> KMAFTLADRVTEEMLADKAALVVEVVEENYHDAPIVGIAVVNEHGRFFLRPETALADPQFVAWLGDETKKKSMFDSKRAAVALKWKGIELCGVSFDLLLAAYLLDPAQGVDDVAAAAKMKQYEAVRPDEAVYGKGAKRAVPDEPVLAEHLVRKAAAIWALERPFLDELRRNEQDRLLVELEQPLSSILAEMEFAGVKVDTKRLEQMGEELAEQLRTVEQRIYELAGQEFNINSPKQLGVILFEKLQLPVLKKS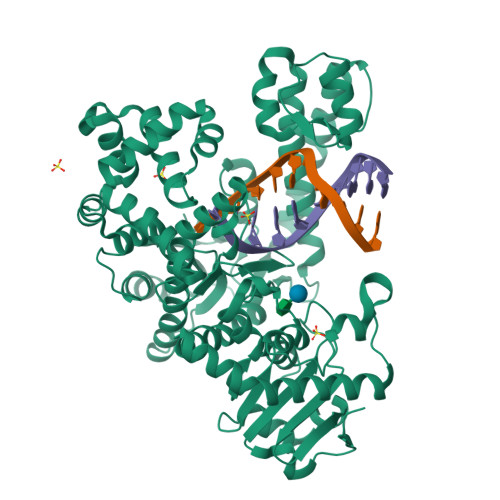KTGYSTSADVLEKLAPYHEIVENILHYRQLGKLQSTYIEGLLKVVRPDTKKVHTIFNQALTQTGRLSSTEPNLQNIPIRLEEGRKIRQAFVPSESDWLIFAADYSQIELRVLAHIAEDDNLMEAFRRDLDIHTKTAMDIFQVSEDEVTPNMRRQAKAVNFGIVYGISDYGLAQNLNISRKEAAEFIERYFESFPGVKRYMENIVQEAKQKGYVTTLLHRRRYLPDITSRNFNVRSFAERMAMNTPIQGSAADIIKKAMIDLNARLKEERLQARLLLQVHDELILEAPKEEMERLCRLVPEVMEQAVTLRVPLKVDYHYGSTWYDAK Human RNA exoribonuclease 2 (Rexo2) is an evolutionarily conserved 3′-to-5′ DEDDh-family exonuclease located primarily in mitochondria. Rexo2 degrades small RNA oligonucleotides of <5 nucleotides (nanoRNA) in a way similar to Escherichia coli Oligoribonuclease (ORN), suggesting that it plays a role in RNA turnover in mitochondria. Rexo2 forms a homodimer and interacts mainly with the last two 3′-end nucleobases of substrates by hydrophobic and π−π stacking interactions via Leu53, Trp96, and Tyr164, signifying its preference in binding and degrading short oligonucleotides without sequence specificity. Rexo2 contains four strictly conserved DEDD residues (D47, E49, D147, D199) for binding two metal ions, as well as a general base (H194) in the active site for hydrolysis of the phosphodiester bonds in nucleic acid substrates.

We obtained three complex cocrystals, referred to as Rexo2–RNA (Rexo2–D199A bound with a 12-nt U12 RNA and Mg2+), Rexo2–DNA1 (wild-type Rexo2 bound with a 5-nt T5 DNA), and Rexo2-DNA2 (Rexo2–D199A bound with a 10-nt T10 DNA and Mg2+). The electron density for DNA oligonucleotides in Rexo2–DNA1 was broken, likely because wild-type Rexo2 was used here for cocrystallization with the partially degraded DNA. In the Rexo2–DNA1 complex, we used wild-type Rexo2 for cocrystallization with DNA in the absence of Mg2+. However, again, we still observed two metal ions (with a low occupancy of 0.81 for MgA and 0.73 for MgB) bound in the active site, likely representing endogenous Mg2+ from the E. coli host strain. In the Rexo2–RNA and Rexo2–DNA1 complexes, only the last two 3′-end nucleotides were observed, i.e., U–U in Rexo2–RNA and T–T in Rexo2–DNA1, with the remainder of the substrates being disordered. Similarly, in Rexo2–DNA1 and Rexo2–DNA2 complex structures, DNA substrates were bound only in the active site of protomer B but not observed in protomer A. Moreover, the 3′-end OH group (O3′) forms a hydrogen bond with the Met50 backbone (NH atom) and Glu49 (Oδ) in all three complexes, providing the structural basis for the preference of Rexo2 for cleaving oligonucleoties with a 3′-OH end. The crystal structures of Rexo2 in complex with DNA reveal a similar DNA oligonucleotide-binding mode to that for RNA.

>[2x]AAGESMAQRMVWVDLEMTGLDIEKDQIIEMACLITDSDLNILAEGPNLIIKQPDELLDSMSDWCKEHHGKSGLTKAVKESTITLQQAEYEFLSFVRQQTPPGLCPLAGNSVHEDKKFLDKYMPQFMKHLHYRIIDVSTVKELCRRWYPEEYEFAPKKAASHRALDDISESIKELQFYRNNIFKKK> GPGGSGGVTEEQVHHIVKQALQ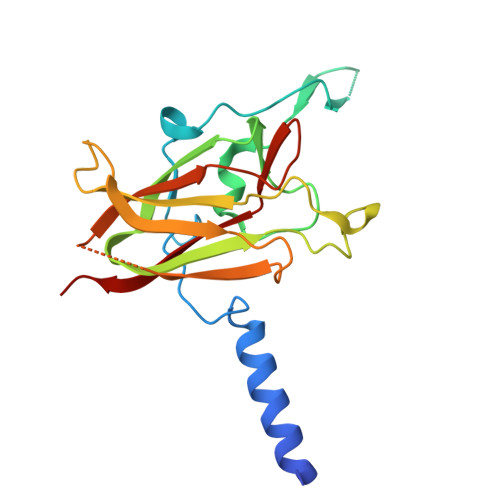RYSEDRIGLADYALESGGASVISTRCSETYETKTALLSLFGIPLWYHSQSPRVILQPDVHPGNCWAFQGPQGFAVVRLSARIRPTAVTLEHVPKALSPNSTISSAPKDFAIFGFDEDLQQEGTLLGKFTYDQDGEPIQTFHFQAPTMGTYQVVELRILTNWGHPEYTCIYRFRVHGEPAH>RVEDLHVGATVAPSSRRDFTFDLYRALASAAPSQNIFFSPVSISMSLAMLSLGAGSSTKMQILEGLGLNLQKSSEKELHRGFQQLLQELNQPRDGFQLSLGNALFTDLVVDLQDTFVSAMKTLYL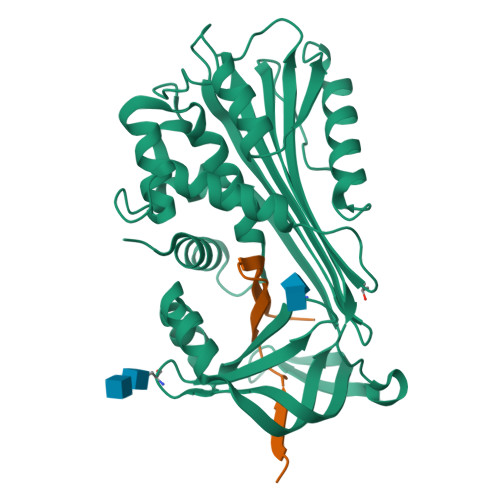ADTFPTNFRDSAGAMKQINDYVAKQTKGKIVDLLKNLDSNAVVIMVNYIFFKAKWETSFNHKGTQEQDFYVTSETVVRVPMMSREDQYHYLLDRNLSCRVVGVPYQGNATALFILPSEGKMQQVENGLSEKTLRKWLKMFKKRQLELYLPKFSIEGSYQLEKVLPSLGISNVFTSHADLSGISNHSNIQVSEMVHKAVVEVDESGTRAAAATGTIFTFRSA[4x];>[4x]RLNSQRLVFNRPFLMFIVDNNILFLGKVNRP> ILVIRKGWLTIN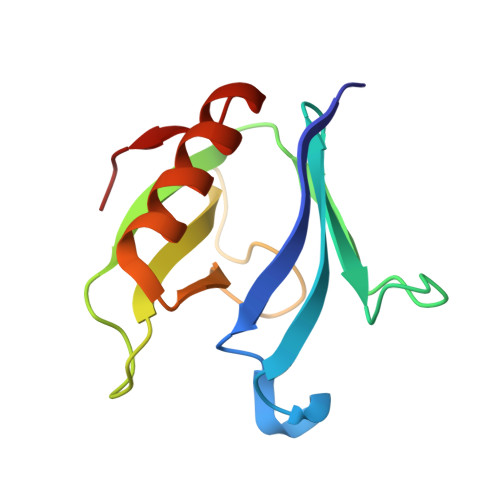NIGIMKGGSKEYWFVLTAENLSWYKDDEEKEKKYMLSVDNLKLRDVEKGFMSSKHIFALFNTEQRNVYKDYRQLELACETQEEVDSWKASFLRAGVYPERV>GSHMTAYTAERQPERDITPVNDETMQEINTL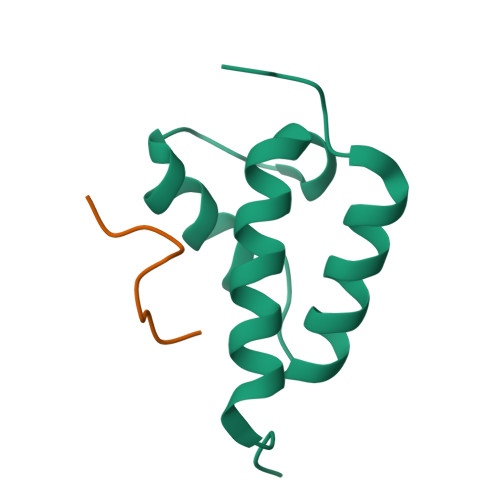LIALDKTWDDDLLPLCSQIFRRDIRASSELTQAEAVKALGFLKQKAAEQKVAA[2x];>[2x]WMDFDDDIPF>QDPCASNPCANGG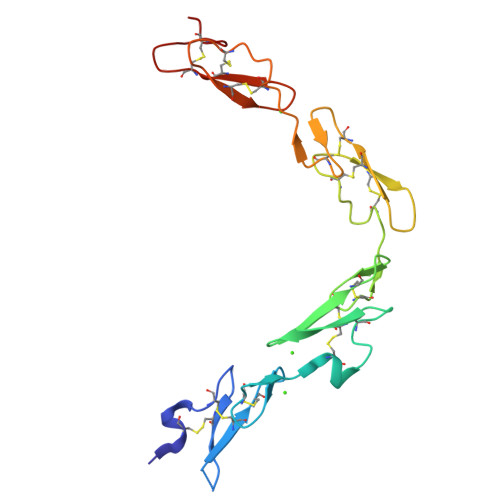QCLPFEASYICHCPPSFHGPTCRQDVNECGEKPGLCRHGGTCHNEVGSYRCVCRATHTGPNCERPYVPCSPSPCQNGGTCRPTGDVTHECACLPGFTGQNCEENIDDCPGNNCKNGGACVDGVNTYNCRCPPEWTGQYCTE[2x]>[3x]MISNAKIARINELA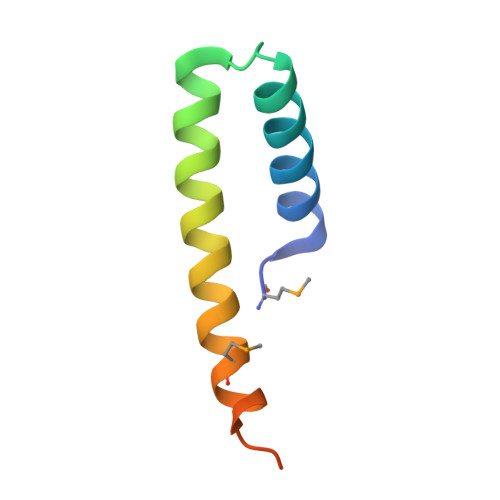AKAKAGVITEEEKAEQQKLRQEYLKGFRSSMKNTLKSVLEHHHHHH(6E)-N-(4-hydroxy-3-methoxybenzyl)-8-methylnon-6-enamide 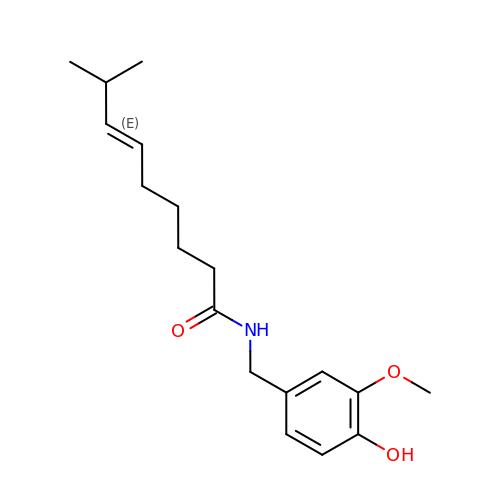| C18 H27 N O3 | YKPUWZUDDOIDPM-SOFGYWHQSA-N> TPRGFVVHTAPVGLA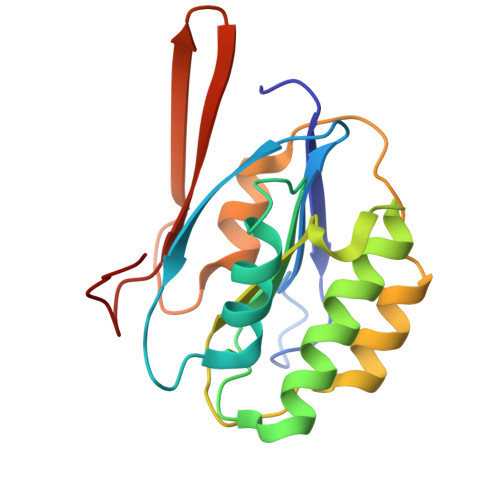DDGRDDFTVLASTAPATVSAVFTRSRFAGPSVVLCREAVADGQARGVVVLARNANVATGLEGEENAREVREAVARALGLPEGEMLIASTGVIGRQYPMESIREHLKTLEWPAGEGGFDRAARAIMTTDTRPKEVRVSVGGATLVGIAKGVGMLEPDMA> ERVNVNLTSIKKLREKVDDSIHRELTDIFANLNYVGVVDEERRLAAIQHDLKLFLIDYGSVCYE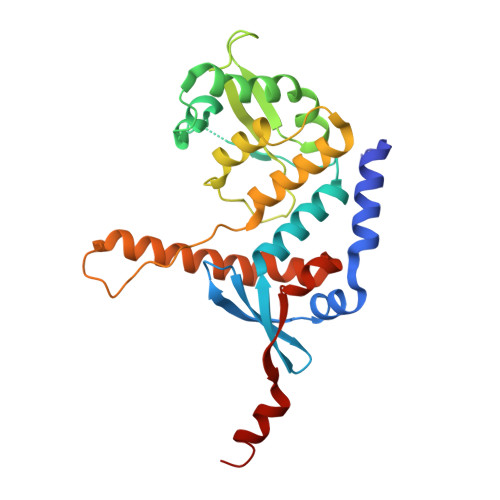LFYQIGLTDFANFGKINLQSTNVSDDIVLYNLLSEFDELNDDASKEKIISKIWDMSSMLNEYYSIELVNDGLDNDLKSVKLKSLPLLLKGYIPSLVKLPFFIYRLGKEVDWEDEQECLDGILREIALLYIPDMVPKVDTSDASLSEDEKAQFINRKEHISSLLEHVLFPCIKRRFLAPRHILKDVVEIANLPDLYKVFERC> GGTCG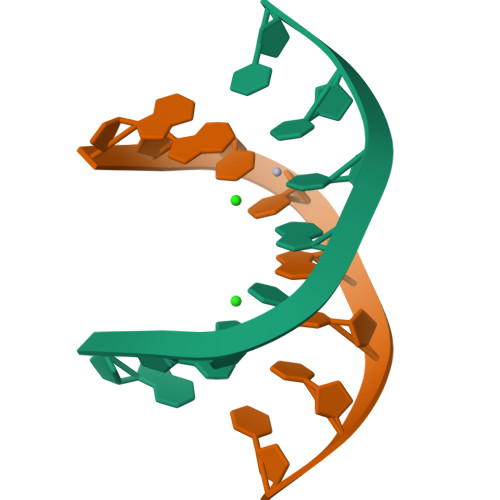TCC>[4x]GPLGSMEKNMRPYTVLWADDEIDLLKPHILFLEQKGYQVTPVLSGNDAIEAVQNNDFDIVFLDENMPGIGGLDALQKIKELKPYTPVVMITKSEEEHIMTQAIGGKIADYLIKPVNPNQLLLSLKKNLQQHSIISETTNTNYRQEFVQLGTQMSGKLSFEEWKELYRRIVFWEIELEQADRQMGELLEMQKQEANRLFARFVTQNYREWIAKPDTRPTMSPDLFKQKVFPLLDNGEKVFFILIDNFRQDQWESVKSMLSEFYTFEEDMYLSILPTATQYARNAIFSGLMPLQIEKMFPDLWVDEESEEGKNLNEEPMIRTLIERYRKHYSFSYNKVY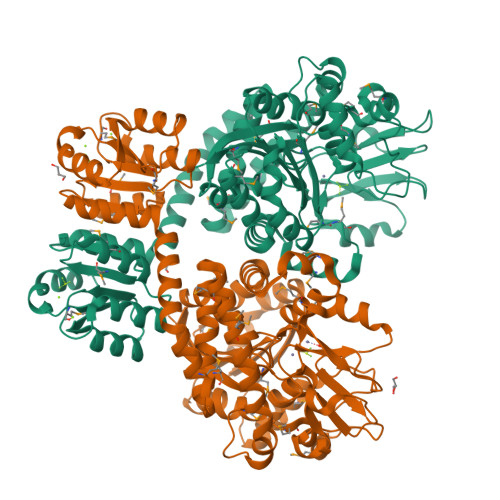ETKFGERLLGQIRSLSQNQLNVIVLNFVDMMSHARTDSKMIRELASNEAAYRSLTKSWFKHSTTYNLFRSIAEMGYKVVLTTDHGTIQVKNPVKVIGDRSTNTNLRYKIGKNLDYNPKEVFEIKDPASVGLPHNNLSDKFIFTKEDDFFAYPNNYNYYVQYYRNTFQHGGISLEEMLVPVITMQPK>[2x]MLYKEPEDGEKIKFDKGKWIVPNKPVILYIEGDGIGPEITNAAIKVINKAVERAYGSSREIKWLEVYAGEKAEKLVNDRFPKETQEMLLKYRVVLKGPLETPIGKGWKSVNVAIRLMLDLYANIRPVKYIEGLESPLKHPEKVDMIIFRENTDDLYRGIEYPFNSEEAKKIR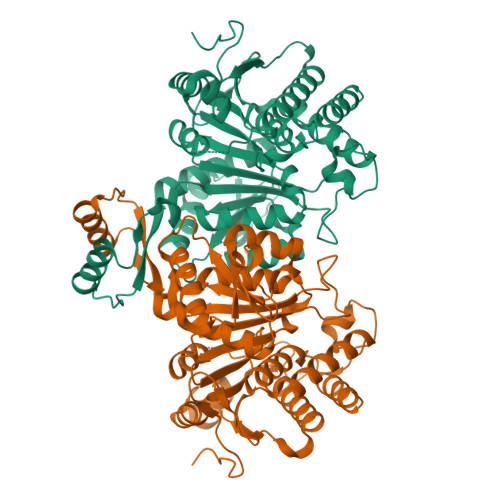DFLRKELKVEIEDDTGIGIKVMSKYKTQRITRLAIQYAIEHKRKKVTIMHKGNVMKYTEGAFREWAYEVALKEYRDFIVTEEEINQGKPDQGKIILNDRIADNMFQQIIIRPEEYDIILAPNVNGDYISDAAGALIGNIGMLGGANIGDEGGMFEAIHGTAPKYAGKNVANPTGIIKAGELMLRWMGWNEAADLIEKAINMAIRDKKVTQDIARFMGVKALGTKEYADELIKIMDTI> IPVIEPLFTKVTEDIPGAQGPVFDKNGDFYIVAPEVEVNGKPAGEILRIDLKTGKKTVICKPEVNGYGGIPAGCQCDRDANQLFVADMRLGLLVVQTDGTFEEIAKKDSEGRRMQGCNDCAFDYEGNLWITAPAGEVAPADYTRSMQEKFGSIYCFTTDGQM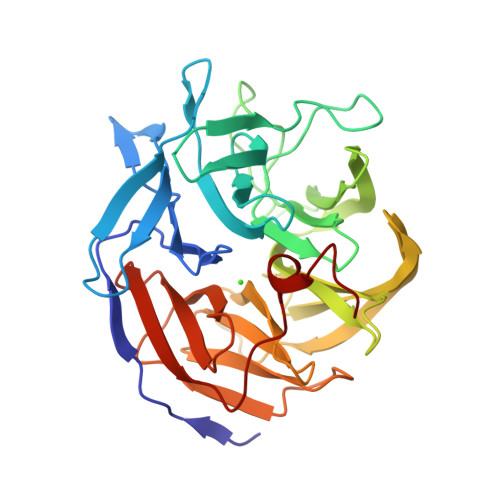IQVDTAFQFPNGIAVRHMNDGRPYQLIVAETPTKKLWSYDIKGPAKIENKKVWGHIPGTHEGGADGMDFDEDNNLLVANWGSSHIEVFGPDGGQPKMRIRCPFEKPSNLHFKPQTKTIFVTEHENNAVWKFEWQRNGKKQYCETLKFGIF FtfL is a key enzyme in C1 metabolism pathway. It catalyzes the synthesis of formyltetrahydrofolic acid from formic acid and tetrahydrofolic acid. Formyltetrahydrofolic acid is then converted through two reactions to 5,10-methylene tetrahydrofolic acid, a metabolite for biosynthesis of pyrimidines and amino acids. PaFtfL exhibits a tetramer in all three crystal structures, consistent with other reported FtfL crystal structures.

To further investigate the structural mechanism of FtfL inhibition by BBR, we determined the crystal structures of PaFtfL apo enzyme, PaFtfL complexed with its substrate ATP, as well as PaFtfL complexed with BBR at 2.0 Å, 2.3 Å, and 2.6 Å resolutions, respectively. Protomers A/B and protomers C/D form two stable dimers with an interface area of 2100 Å2, and the two dimers assemble into a tetramer with an additional interface area of 620 Å2. Each protomer comprises its own solvent-exposed active site close to the protomer interface. Structural comparison reveals that PaFtfL adopts essentially the same overall fold for each of the protomers and exhibits an identical active site as in reported crystal structures of FtfL from other bacterial species, indicative its conserved catalytic mechanism.

>[4x]GSHMMEFKTDIEIAQEANPQDIRDIAKKINLSEDDIELYGKYKAKIDYNVLNRTKSRAGKLILTTAINPTPAGEGKTTTSIGVADALAKLGKNVIAALREPSMGPVFGIKGGAAGGGYAQVVPMEDINLHFTGDMHAIGAANNLLAAMLDNHVYQTNSLNINPKRITWRRCVDMNDRQLRNVVDGLGKKVDGVTREDGFDITVASEVMAAFCLSNNISELKENLGNIVVAYNYSGKPVTARDLNAHGAMAAILKDALKPNLVQTLEGTPAILHGGPFANIAHGCNSIIATKMGMHMADYVVTEAGFGADLGAEKFLDIKCRKAGIRPDAVIIVATVRALKYNGGVAKDQLNNENLEALEKGLPNLLKHIENITQVYKIPAVVAINRFPLDTDAELALVRSKCEELGVKVALSEVWANGGEGGIEVANEVLKLIEEGENNFEYCYEEDMTIKEKLNAIATKIYGADGVNYTKEANKQIAELEELGFGNLPVCVAKTQYSLSDDQTKLGRPTGFTIEVRQANISAGAGFVVVMTGEIMKMPGLPKLPAAERIDVDENGKISGLF>SAEHVLTMLNEHEVKFVDLRFTDTKGKEQHVTIPAHQVNAEFFEEGKMFDGSSIGGWKGINESDMVLMPDASTAVIDPFFADSTLIIRCDILEPGTLQGYDRDPRSIAKRAEDYLRATGIADTVLFGPEPEFFLFDDIRFGASISGSHVAIDDIEGAWNSSTKYEGGNKGHRPGVKGGYFPVPPVDSAQDIRSEMCLVMEQMGLVVEAHHHEVATAGQNEVATRFNTMTKKADEIQIYKYVVHNVAHRFGKTATFMPKPMFGDNGSGMHCHMSLAKNGTNLFSGDKYAGLSEQALYYIGGVIKHAKAINALANPTTNSYKRLVPGYEAPVMLAYSARNRSASIRIPVVASPKARRIEVRFPD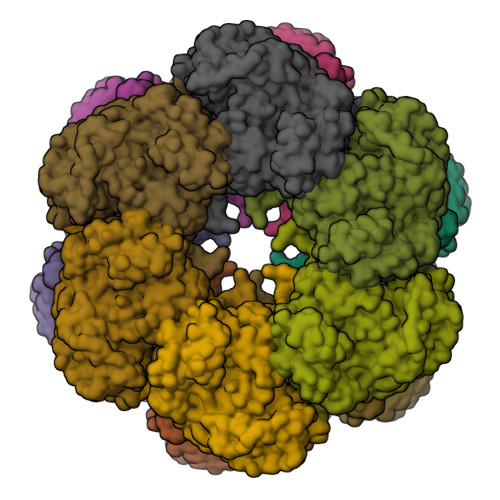PAANPYLCFAALLMAGLDGIKNKIHPGEPMDKNLYDLPPEEAKEIPQVAGSLEEALNALDLDREFLKAGGVFTDEAIDAYIALRREEDDRVRMTPHPVEFELYYSV[12x]> MSELEKAVVALIDVFHQYSGREGDKHKLKKSELKELINNELSHFLEEIKEQEVVDKVMETLDSDGDGECDFQEFMAFVAMITTACHEFF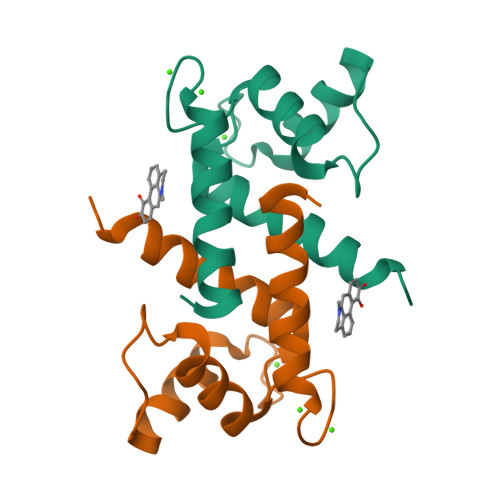EHE>[4x]MRAAVVYKTDGHVK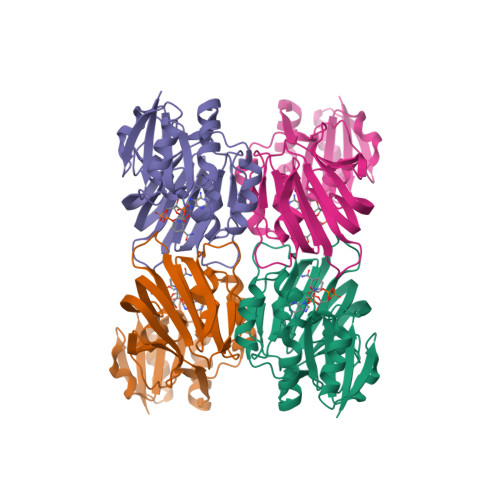RIEEALKRLEVEVELFNQPSEELENFDFIVSVGGDGTILRILQKLKRCPPIFGINTGRVGLLTHASPENFEVELKKAVEKFEVERFPRVSCSAMPDVLALNEIAVLSRKPAKMIDVALRVDGVEVDRIRCDGFIVATQIGSTGYAFSAGGPVVEPYLECFILIPIAPFRFGWKPYVVSMERKIEVIAEKAIVVADGQKSVDFDGEITIEKSEFPAVFFKNEKRFRNLFGKVRSIG>[2x]MD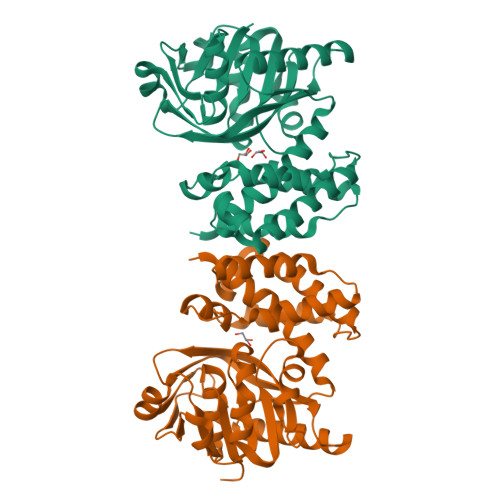SKQQRIGVIGTGAIGGFYGLMLAHAGHDVHFLLRSEFEAVNRAGLSLNSAVHGFRRLAPVQAYHSAQDMPPCDWLLVGAKTTGNHELAPLIRAAAAPGAKVLLLQNGLGVEERLRPLLPESLHLLGGLCFICVHRGEPGVIEHQAYGGVNLGYHSGPADERRRREIVEEGAALFRESGLESTAMPDLEQARWQKLVWNIPYNGLSVLLKSSTAPLMANADSRSLIEAIMEEVIGAAGACGFILPEGYADQLLAATERMPDYRPSMYHDFAHGRPLELAAIYAAPLARAAAAGYRMPRVEALHQALRFLEAQPR> NHPMLMNL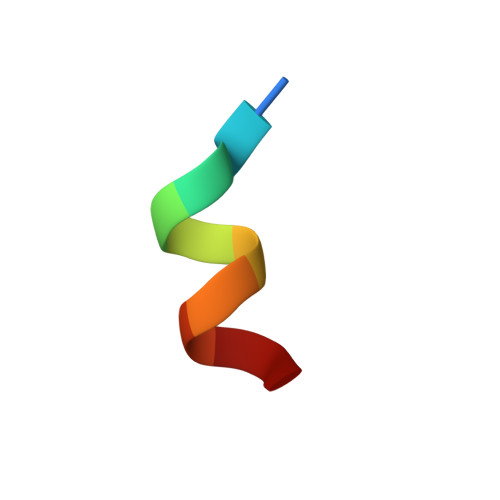LK>[2x]GPGSPAASKSDKLAATPGMFVQHSTAAFSDRYKGQRVLGKGSFGEVILCKDKVTGQEYAVKVISKRQVKQKTDKELLLKEVELLKKLDHPNIMKLYEFFEDKGYFYLVTEVYTGGELFDEIISRKRFSEVDAARIIRQVLSGITYMHKNKIVHRDLKPENLLLENKRKD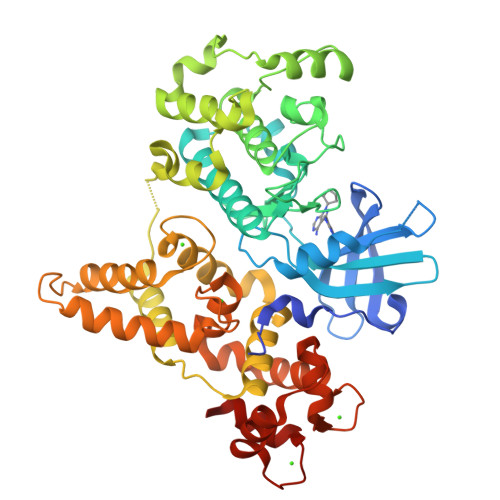ANIRIIDFGLSTHFESTKKMKDKIGTAYYIAPEVLHGTYDEKCDVWSTGVILYILLSGCPPFNGANEFDILKKVEKGKFTFDLPQWKKVSEPAKDLIRKMLAYVPTMRISARDALEHEWLKTTDAATDSIDVPSLESTILNIRQFQGTQKLAAAALLYMGSKLTTNEETVELNKIFQRMDKNGDGQLDKQELMEGYVELMKLKGEDVSALDQSAIEFEVEQVLDAVDFDKNGFIEYSEFVTVAMDRKTLLSRQRLERAFGMFDADGSGKISSSELATIFGVSEVDSETWRRVLAEVDRNNDGEVDFEEFRQMLLKLCGDTAA> GEFELMEMILEEKDASDWIYRGEGGANLVLAYAGSSPLFVGKVIRIQKARRNDKAIKNSNGVVSVLTSDEQHLWRENNELISSPNKEVLEQRYVQNVIIPLLGPKHVDAGVRVSVSKEFLECVDKKVTKQRPLWRVNAANVDTSHDSALILNDHSLFSQGITSGGDCISVEIKPKCGFLPTSRFIGKENMLKTSVSRFKMHQLLKLEYIEISEESEYDPLDLFSGSKERVLEAIKALYSTPQNNFRVFLNGSLILG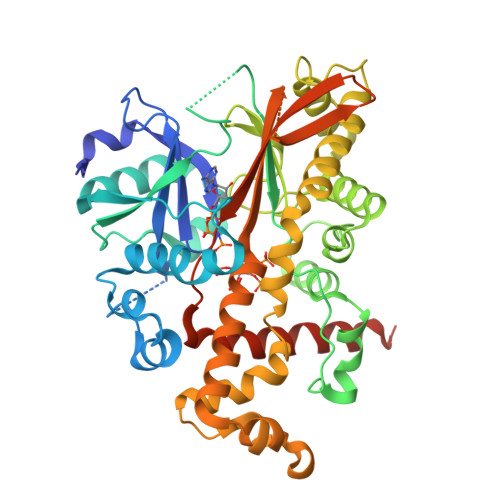GSGESTGRTSPEIGYAFEDALKGFIQSEDGHRTECFLQLVSDAVYGSGVLDRLLEIQKLDKLDIEGAIHCYYDIINQPCPICREGRPLEAELSLHALPLDESLKIVKEYLIAATAKDCSIMISFQSRNAWDSEPSGDYVSLKPTNQTFDYKVHFIDLSLKPLKRMESYYKLDKKIISFYNRKQKAENTAEQIGNSKPSHS>MSSGTPTPSNVV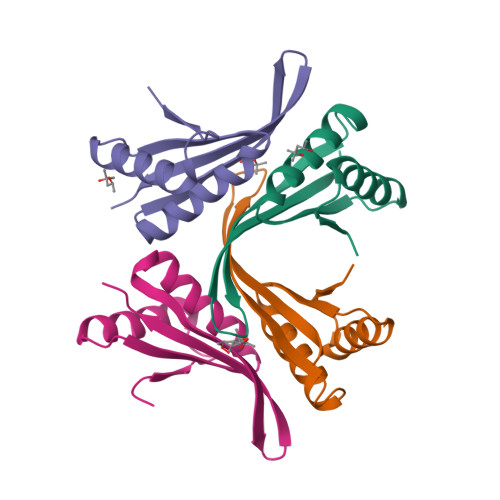LIGKKPVMNYVLAALTLLNQGVSEIVIKARGRAISKAVDTVEIVRNRFLPDKIEIKEIRVGSQVVTSQDGRQSRVSTIEIAIRKK[2x];>MTEKLNEIVVRKTKNVEDHVLDVIVLFNQGIDEVILKGTGREISKAVDVYNSLKDRLGDGVQLVNVQTGSEVRDRRRISYILLRLKRVY[2x]>[4x]MNSQQNPDLAVHPLAIPMEGLLGESATTLEKNVIATQLSEEAQVKLEVIQSLLEPCDRTTYGQKLREAAEKLNVSLRTVQRLVKNWEQDGLVGLTQTSRADKGKHRIGEFWENFITKTYKEGNKGSKRMTPKQVALRVEAKARELKDSKPPNYKTVLRVLAPILEKQQKAKSIRSPGWRGTTLSVKTREGKDLSVDYSNHVWQCDHTRVDVLLVDQHGEILSRPWLTTVIDTYSRCIMGINLGFDAPSSGVVALALRHAILPKRYGSEYKLHCEWGTYGKPEHFYTDGGKDFRSNHL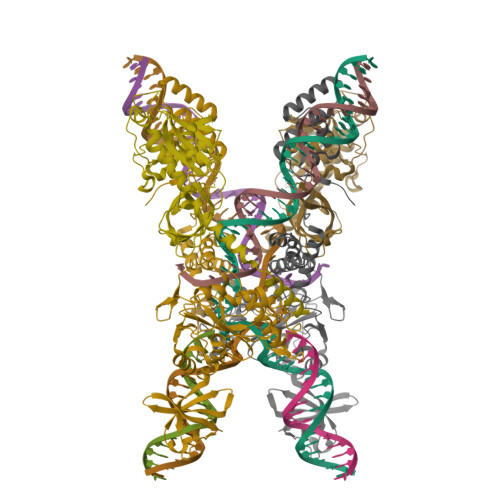SQIGAQLGFVCHLRDRPSEGGVVERPFKTLNDQLFSTLPGYTGSNVQERPEDAEKDARLTLRELEQLLVRYIVDRYNQSIDARMGDQTRFERWEAGLPTVPVPIPERDLDICLMKQSRRTVQRGGCLQFQNLMYRGEYLAGYAGETVNLRFDPRDITTILVYRQENNQEVFLTRAHAQGLETEQLALDEAEAASRRLRTAGKTISNQSLLQEVVDRDALVATKKSRKERQKLEQTVLRSAAVDESNRESLPSQIVEPDEVESTETVHSQYEDIEVWDYEQLREEYGF> EEATFTANFKDTDLKSFIETVGANLNKTIIMGPGVQGKVSIRTMTPLNERQYYQLFLNLLEAQGYAVVPMENDVLKVVKSSAAKVEPLPLVGEGSDNYAGDEMVTKVVPVRNVSVRELAPILRQMIDSAGSGNVVNYDPSNVIMLTGRASVVERLTEVIQRVDHAGNRTEEVIPLDNASASEIARVLESLTKNSGENQPATLKSQIVADERTNSVIVSGDPATRDKMRRLIRRLDSEMERSGNSQVFYLK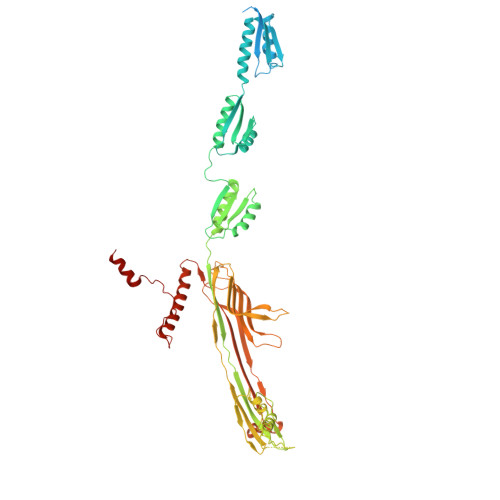YSKAEDLVDVLKQVSGTLTAAKEEAEGTVGSGREIVSIAASKHSNALIVTAPQDIMQSLQSVIEQLDIRRAQVHVEALIVEVAEGSNINFGVQWASKDAGLMQFANGTQIPIGTLGAAISQAKPQKGSTVISENGATTINPDTNGDLSTLAQLLSGFSGTAVGVVKGDWMALVQAVKNDSSSNVLSTPSITTLDNQEAFFMVGQDVPVLTGSTVGSNNSNPFNTVERKKVGIMLKVTPQINEGNAVQMVIEQEVSKVEGQTSLDVVFGERKLKTTVLANDGELIVLGGLMDDQAGESVAKVPLLGDIPLIGNLFKSTADKKEKRNLMVFIRPTILRDGMAADGVSQRKYNYMRAEQIYRDEQGLSLMPHTAQPVLPAQNQALPPEVRAFLNAGRTR>MIKKIGVLTSGGDAPGMNAAIRGVVRSALTEGLEVMGIYDGYLGLYEDRMVQLDRYSVSDMINRGGTFLGSARFPEFRDENIRAVAIENLKKRGIDALVVIGGDGSYMGAMRLTEMGFPCIGLPGTIDNDIKGTDYTIGFFTALS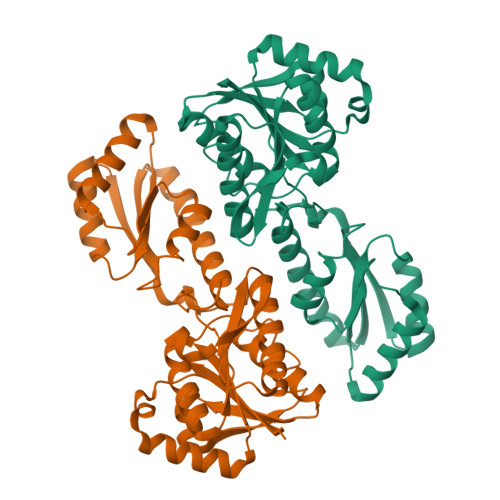TVVEAIDRLRDTSSSHQRISVVEVMGRYCGDLTLAAAIAGGCEFVVVPEVEFSREDLVNEIKAGIAKGKKHAIVAITEHMCDVDELAHFIEKETGRETRATVLGHIQRGGSPVPYDRILASRMGAYAIDLLLAGYGGRCVGIQNEQLVHHDIIDAIENMKRPFKGDWLDCAKKLY[4x]(2E,6Z)-3,7,11-trimethyldodeca-2,6,10-trien-1-yl 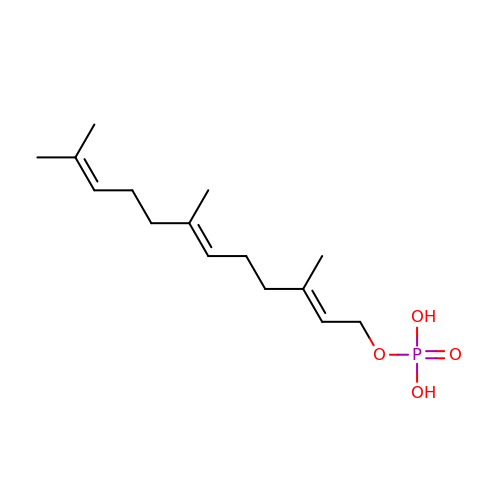dihydrogen phosphate | C15 H27 O4 P | ALEWCKXBHSDCCT-GNESMGCMSA-N>NLFQFAKMINGKLGAFSVWNYISYGCYCGWGGQGTPKDATDRCCFVHDCCYGRVRGCNPKLAIYAYSFKKGNIVCGKNNGCLRDICECDRVAANCFHQNQNTYNKNYKFLSSSRCRQTSEQ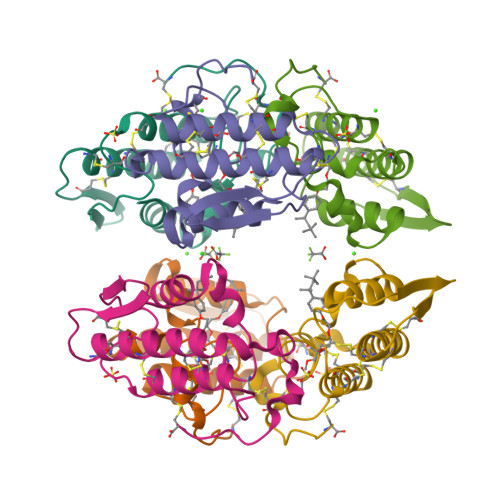C[2x]Evidence indicates that variable lymphocyte receptors (VLRs) play roles equivalent to those of Igs and TCRs in the adaptive immune system of cyclostomes. VLRs consist of an N-terminal cap (LRRNT), the first LRR (LRR1), multiple (usually up to seven) 24-residue variable LRRs (LRRVs), a terminal or end LRRV (LRRVe), a connecting peptide (CP) and a C-terminal cap (LRRCT), followed by an invariant 3′-terminal region. Recently, a third VLR, designated VLRC, was identified in lampreys. VLRC sequences are more closely related to VLRA than to VLRB sequences, leading to the speculation that VLRC+ cells are T-lineage cells and that, like jawed vertebrates equipped with two lineages of T-cells (αβ and γδ T-cells) and one lineage of B-cells, lampreys may have two lineages of T-like cells (analogous to αβ and γδ T-cells) and one lineage of B-like cells.

The crystal structure of the lamprey VLRC ectodomain (residues from His25 to Cys247) was determined by molecular replacement at a resolution of 2.3 Å. The structure has a horseshoe-like solenoid conformation, which is typical of proteins that belong to the LRR protein family. Lamprey VLRC is composed of eight modules, including LRRNT, LRR1, LRRV1, LRRV2, LRRV3, LRRVe, CP and LRRCT in this order. The concave surface of lamprey VLRC is formed by the β-sheet made up of eight β-strands (two from LRRNT, five from LRRs and one from CP); the β1-strand is anti-parallel whereas the remaining β-strands are arranged in a parallel fashion. Like VLRA and VLRB, N-terminal and C-terminal caps of VLRC have a total of four disulfide bonds presumably important for structural integrity: two within the LRRNT (Cys28-Cys39, Cys37-Cys52) and two within the LRRCT (Cys200-Cys227, Cys202-Cys247). We calculated the Shannon entropy for each position based on the multiple alignments of 102 Japanese lamprey VLRC sequences and mapped variable residues onto the VLRC crystal structure. This revealed that variable residues are located predominantly on the concave surface, in particular in the region around the core β-sheet, suggesting that, similar to VLRA and VLRB, VLRC recognizes its ligands through the concave surface. A striking feature of lamprey VLRC is that its N-terminal cap has a long loop protruding toward the concave surface. This protrusion is formed by amino acid residues 41–48 located in the region connecting two β-strands β1 and β2. Indeed, ∼80% of known VLRC sequences from Lethenteron japonicum have the same sequence, NKTDSSPE, and the remaining ∼20% have closely related sequences. Crystallographic analysis of VLRC confirmed this prediction.

> MNHKHHHHHHHHHHSSGENLYFQGHMACLAVGKDDICTCSNKTDSSPETVDCSSKKLTAVPTGIPANTEKLQLDFNQLANIPAEAFHGLTRLTYLALDYNQLQSLPVGVFDQLNNLNELRLQDNQLTSLPPGVFDSLTKLTYLTLSQNQLQSIPAGVFDKLTNLNRLELSTNQLQSVPHGAFDSLVNLETLHLELNPWDCACSDIIYLRTFIAKNTDKISGMESAQCNGTSTAVKDVNTEKIKNVTCN> GSMDPAIYFKEQFLDGDAWTNRWVESKHKSDFGKFVLSSGKFYGDLEKDKGLQTSQDARFYALSAKFEPFSNKGQTLVVQFT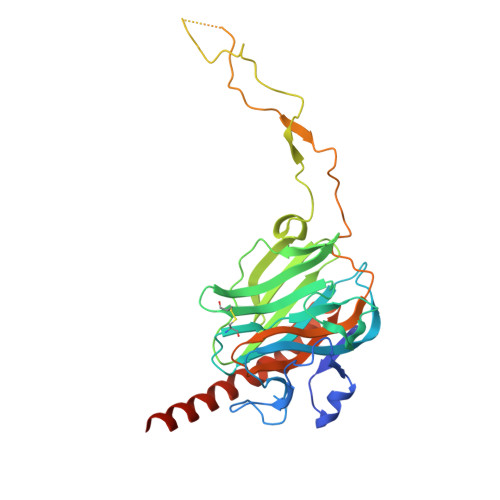VKHEQNIDCGGGYVKLFPSGLDQKDMHGDSEYNIMFGPDICGPGTKKVHVIFNYKGKNVLINKDIRSKDDEFTHLYTLIVRPDNTYEVKIDNSQVESGSLEDDWDFLPPKKIKDPDAAKPEDWDERAKIDDPTDSKPEDWDKGGSGGEWKPRQIDNPDYKGTWIHPEIDNPEYSPDANIYAYDSFAVLGLDLWQVKSGTIFDNFLITNDEAYAEEFGNETWGVTKAAEKQMKDKQDEEQRLKLEHHHHHH> GAMGIVGVGIDLVSIPDFAEQVDQPGTVFAETFTPGERRDASDKSSSAARHLAARWAAKEAVIKAWSGSRFAQRPVLPEDIHRDIEVVTDMWGRPRVRLTGAIAEYLADVTIHVSLTHEGDTAAAVA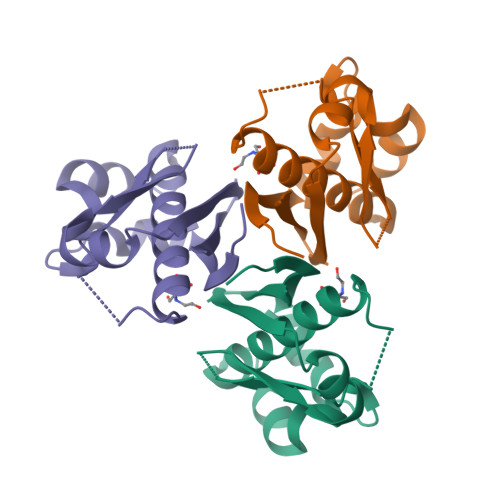ILEAP4-(6-{[(1S)-1-(HYDROXYMETHYL)-2-METHYLPROPYL]AMINO}IMIDAZO[1,2-B]PYRIDAZIN-3-YL)BENZONITRILE | 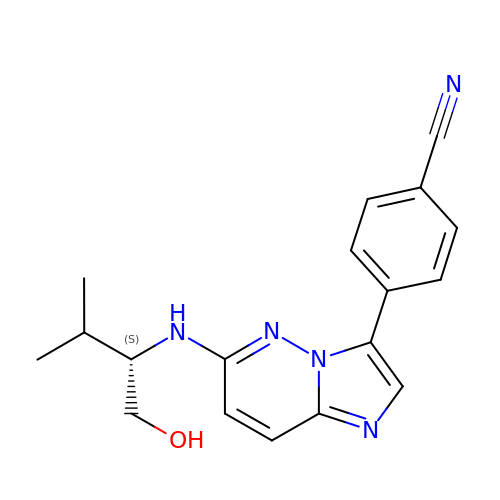C18 H19 N5 O | CQZVJEKKNHOFNB-OAHLLOKOSA-N>[2x]PKIVVVGAVAGGATC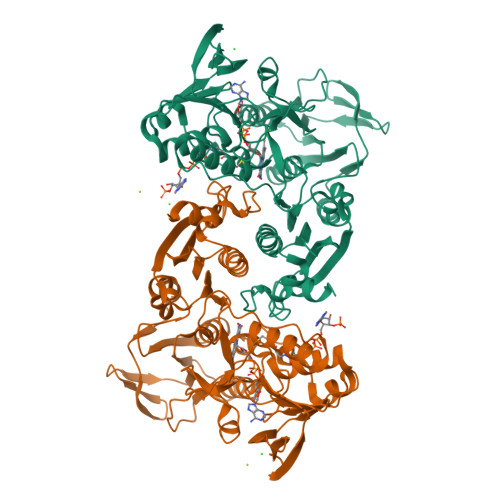ASQIRRLDKESDIIIFEKDRDMSFANCALPYVIGEVVEDRRYALAYTPEKFYDRKQITVKTYHEVIAINDERQTVSVLNRKTNEQFEESYDKLILSPGASANSLGFESDITFTLRNLEDTDAIDQFIKANQVDKVLVVGAGYVSLEVLENLYERGLHPTLIHRSDKINKLMDADMNQPILDELDKREIPYRLNEEINAINGNEITFKSGKVEHYDMIIEGVGTHPNSKFIESSNIKLDRKGFIPVNDKFETNVPNIYAIGDIATSHYRHVDLPASVPLAWGAHRAASIVAEQIAGNDTIEFKGFLGNNIVKFFDYTFASVGVKPNELKQFDYKMVEVTQGAHANFYPGNSPLHLRVYYDTSNRQILRAAAVGKEGADKRIDVLSMAMMNQLTVDELTEFEVAYAPPYSHPKDLINMIGYKAK NsP1 is the membrane anchor for the complex, forming dodecameric pores that associate monotopically with the membrane in the necks of the spherules to gate their entrance. Enzymatically, nsP1 also has a role in addition of cap0 structures to the 5′ end of the positive-sense viral RNAs. NsP1 possesses both N′7 methyltransferase and guanylyltransferase activity and reverses the order of these reactions. Each nsP1 protomer is built around a methyltransferase fold common to SAM-dependent methyltransferases with additional insertions (membrane binding and oligomerisation (MBO) loops 1 and 2) and extensions (ring aperture membrane binding oligomerisation (RAMBO) domain) that contribute to pore formation, oligomerization, and membrane binding.

In order to investigate the structure of the pores after the capping/decapping reaction, we analyzed by cryo-EM the structure of nsP1 pores incubated with a cap0 11-nucleotide-long CHIKV RNA. However, after the decapping reaction, we could distinguish two different three-dimensional (3D) classes; one similar to the previous structures and a second with significant changes in the first 130 residues and the C-terminal alpha helix k of nsP1. Electron density for the m7GMP base was found in the GTP binding site in both classes. The nsP1 protomers appear tilted outward 8° with respect to the equatorial axis of the ring. The pore opening results on an increase of the inner aperture of 3 Å (from 70 to 73 Å) and the outer diameter of 12 Å (from 178 Å to 190 Å) and a change in the surface charge distribution concomitant with a projection of the active site toward the top of the ring. This conformation resembles the structure of nsP1 pores when expressed in mammalian cells (Discussion) (13), and was not observed in datasets of m7GMP–nsP1 produced following incubation of the substrates and uncapped RNA. Thus, we can conclude that the decapping reaction induces a motion in the ring resulting in an opening of the pore aperture. Here, we show how the postdecapping state induces motions that trigger an opening in the pore, similar to the open form of nsP1 complexes expressed in mammalian cells. This open form increases surface exposure of the RNA binding pockets, with a concomitant redistribution of surface charges along a path leading to the internal pore.

>[12x]MDPVYVDIDADSAFLKALQRAYPMFEVEPRQVTPNDHANARAFSHLAIKLIEQEIDPDSTILDIGSAPARRMMSDRKYHCVCPMRSAEDPERLANYARKLASAAGKVLDRNISGKIGDLQAVMAVPDTETPTFCLHTDVSCRQRADVAIYQDVYAVHAPTSLYHQAIKGVRLAYWVGFDTTPFMYNAMAGAYPSYSTNWADEQVLKAKNIGLCSTDLTEGRRGKLSIMRGKKLEPCDRVLFSVGSTLYPESRKLLKSWHLPSVFHLKGKLSFTCRCDTVVSCEGYVVKRITMSPGLYGKTTGYAVTHHADGFLMCKTTDTVDGERVSFSVCTYVPATICDQMTGILATEVTPEDAQKLLVGLNQRIVVNGRTQRNTNTMKNYMIPVVAQAFSKWAKECRKDMEDEKLLGVRERTLTCCCLWAFKKQKTHTVYKRPDTQSIQKVQAEFDSFVVPSLWSSGLSIPLRTRIKWLLSKVPKTDLTPYSGDAQEARDAEKEAEEEREAELTLEALPPLQAAQEDVQVEIDVEQLEDRAGA>SMACYGGFDLYFILDKSGSVLHHWNEIYYFVEQLAHKFISPQLRMSFIVFSTRGTTLMKLTEDREQIRQGLEELQKVLPGGDTYMHEGFERASEQIYYENRQGYRTASVIIALTDGELHEDLFFYSEREANRSRDLGAIVYAVGVKDFNETQLARIADSKDHVFPVNDGFQALQGIIHSILKKSC[6x]

By using a genetic approach, two PA cell surface receptors have been identified: TEM8/ANTXR1 (tumor endothelial marker 8/anthrax toxin receptor 1) and CMG2/ANTXR2 (capillary morphogenesis protein 2/anthrax toxin receptor 2). TEM8 and CMG2 are type I transmembrane proteins with three domains: an N-terminal, extracellular von Willebrand factor type A domain (vWA domain), a single transmembrane spanning domain, and a C-terminal cytosolic domain. CMG2 was reported to have approximately 1000-fold higher affinity for PA (Kd = 170 and 780 pM for the Mg2+- and Ca2+-bound complexes, respectively) than TEM8 (Kd = 1.1 µM and 130 nM for the Mg2+- and Ca2+-bound complexes, respectively), the latter of which is about the average level of integrin-ligand interaction. The MIDAS (metal ion-dependent adhesion site) motif in vWA domains can exist in either of two conformations, much like the integrin I domain: closed (low-affinity ligand binding state) and open (high-affinity ligand binding state).

Here we report the high resolution structure of the TEM8 vWA domain. We found that the vWA domain contains a chelated Mg2+ ion and a bound pseudo-ligand (i.e., an acetate ion from the crystallization buffer) in its MIDAS site. Our crystal structure contained six TEM8 vWA molecules (labeled as A, B, C, D, E, and F) in the asymmetric unit (also unit cell). Three monomers were related by a non-crystallographic three-fold symmetry to form a trimer, and two of such trimers (A-B-C and D-E-F) formed a hexamer with an overall ball-like shape through a two-fold axis perpendicular to the three-fold axis. In this hexamer, the MIDAS ligand binding area from each monomer was blocked, which would definitely interrupt the interaction between TEM8 and PA. Thus, the observed TEM8 hexamer is most likely an artifact of crystal packing. Consistent with their sequence homology, the structure of the TEM8 extracellular domain is very similar to that of CMG2 and the integrin A domain. It should be noted that three acetate ions were found in each of the six TEM8 molecules and were well defined in the electron density map. One of them appeared to correspond to an analogous ion in the CMG2 structure, which acted as a mimic ligand of the side chain of D683 in PA and occupied the MIDAS coordination site. Taken together, the TEM8 extracellular domain contained a conserved Mg2+-coordinated MIDAS motif that assumed an integrin-like open conformation.>MDNKNNKPTDQEILKTSRAVGEIPSADNLKNRFKARSIPLETDFTNLIDLAEVGRLAIGQSPSQQSKTPGTGMELTSDGKLQVKAGAGVDIDNNNRITIKSGHGIKVDGNGISVKPGSGIKVDSNGVNVNIDDFWEEIRNKIMPKGTMLPIYGTPNPSALPTGWEWCDGKDGRPNLKKGKYNLLSGQSSGTDTFWADNKNGD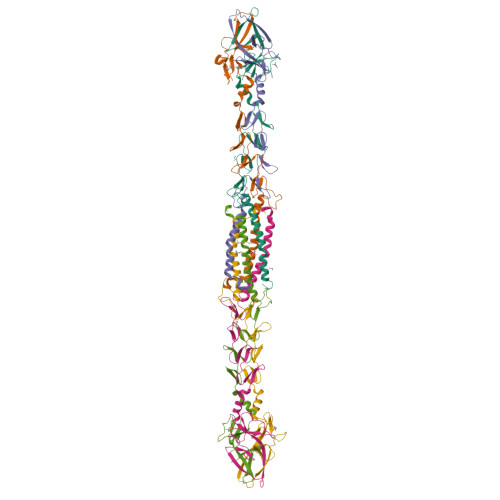TEINVLFVYYMIKVV[6x]1-{(1R,2S)-2-HYDROXY-1-[2-(1-NAPHTHYL)ETHYL]PROPYL}-1H-IMIDAZOLE-4-CARBOXAMIDE | C19 H21 N3 O2 | 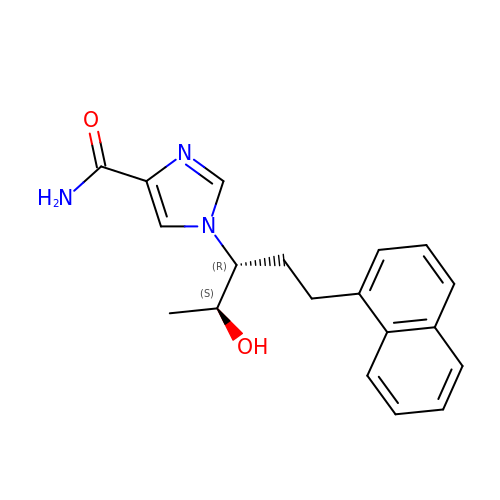OODDZQQDDOVCFD-SCLBCKFNSA-N> GGSGGSGGSGGSGGSPTNYEYDEASETWPSFILTGLLMVVGPMTLLQIYQIFFGANAEDGNSGKSKEFNEEVFKNLNEEYTSDEIKQFRRKFDKNSNKKSKIWSRRNIIIIVGWILVAILLQRINSNDAIKDAATKLFDPYEILGISTSASDRDIKSAYRKLSVKFHPDKLAKGLTPDEKSVMEETYVQITKAYESLTDELVRQNYLKYGHPDGPQSTSHGIASGSGGSGGSASPLLVVCYVALLGLILPYFVSRWWARTQSYTKKGIHNVTASNFVSNLVNYKPSEIVTTDLILHWLSFAHEFKQFFPDLQPTDFEKLLQDHINRRDSGKLNNAKFRIVAKCHSLLHGLLDIACGFRNLDIALGAINTFKCIVQAVPLTPNCQILQLPNVDKEHFITKTGDIHTLGKLFTLEDAKIGEVLGIKDQAKLNETLRVASHIPNLKIIKADFLVPGRPYISLKVLVRSAKQPLIPTSLIPEENLTEPQDSESQ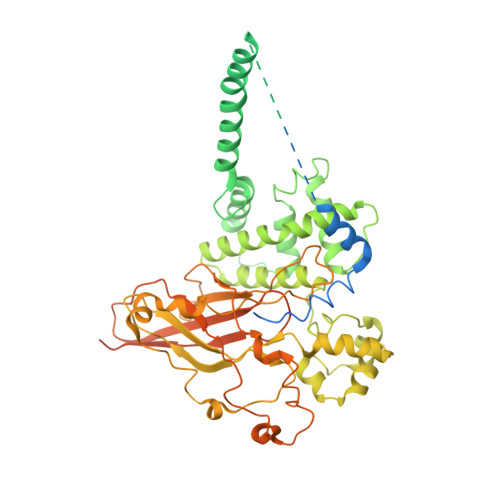RDPFAMMSKQPLVPYSFAPFFPTKRRGSWCCLVSSQKDGKILQTPIIIEKLSYKNLNDDKDFFDKRIKMDLTKHEKFDINDWEIGTIKIPLGQPAPETVGDFFFRVIVKSTDYFTTDLDITMNMKVRDSPAVEQVEVYSEEDDEYSTDDDETESDDESDASDYTDIDTDTEAEDDESPEGENLYFQ> MASATLPRFDLMGWDKKDIADPYPVYRRYREAAPVHRTASGPGKPDTYYVFTYDDVVRVLSNRRLGRNARVASGDTDTAPVPIPTEHRALRTVV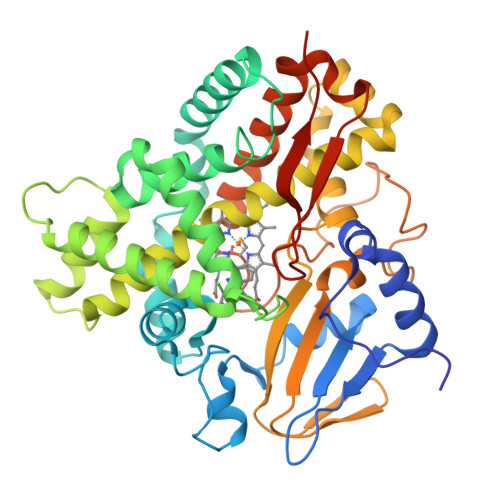ENWLVFLDPPHHTELRSLLTTEFSPSIVTGLRPRIAELASALLDRLRAQRRPDLVEGFAAPLPILVISALLGIPEEDHTWLRANAVALQEASTTRARDGRGYARAEAASQEFTRYFRREVDRRGGDDRDDLLTLLVRARDTGSPLSVDGIVGTCVHLLTAGHETTTNFLAKAVLTLRAHRDVLDELRTTPESTPAAVEELMRYDPPVQAVTRWAYEDIRLGDHDIPRGSRVVALLGSANRDPARFPDPDVLDVHRAAERQVGFGLGIHYCLGATLARAEAEIGLRALLDGIPALGRGAHEVEYADDMVFHGPTRLLLDLPDAALEHHHHHH>MDQITRILEKLNQQRSGETTVTLADFMPMSLAEIRSQNTGRLSREEAQLLHRAAQKEKQNNILYTARMLTRANPLLKKEMNTARYYGATPYGYDDIIPPRAEKFVAPGAVSSMFSPAGYLTELYREARGLHPKDSDRNLDKRRQDLAKLVLSQDNLDNEISALSLANEQLETALMAQTGKTDKNKYYETLATSRRSGVTPYNAPFEGIHNALAQRNFVLPDNILSNPAKFAILAAYDAGISPKLYNILTEDTESLTGSDLENSLKRNFPKVKIKDLMTLDALANYYELPADDIQALIAAEITGRLPTPDVYNDDNKLVIPAINTGGKITFSELAKTQSDEKQADYIDLIPQGGNQFLVNFSVKKTKKDATHFSIGYNKSFNNLADKNGFVPLAGEHYSIPVTLDAKILEKKTKIGITRKKPEPASDENHYTSATFTIHPNAEPGIWLLRLNKTLRLAKVSGMTPHETQHALIHVRNDSSEYELRRFTETLLYRKRYGIDTETALMLCNAGISRISYDGQLSHFDRLFNNPPLNGVTYTLGGDDILMEPDAGDPRREVLKRAFRVDNTGLWQLLVITNRENKSKTIENKTEKLRGLLFVRLLADVHNLTVAQLDALLQISPYNSMNVYALDGKTRQKMLSFLSRITQWLNTQNITVEQLMLLLDKISPAAPTKEMQVLLDLLRNGGIDKTNTKTLYTTMAPVITAAMQLDITESGEALLRWLDNNHPAGILTTSEARKLIIKKGQTAGDKEKLAAWCQALAQRVLVIRTFTLSNAELQTLSQGAPAGTITELYNISDFHNLINRCGEQAGTVLDALQSGTLTVKILAQALNLSEEVITQALTLAGQKPELTTWAQLAVLPPRLDLADTLHITPKDITTLLTVSENVRPFYTDLSALAGLLQAGLNEQQTKQLQNQSEPRRNEALSGEYRSLVMNNPVADRDDIWRNLLVDGKVSAEITTTLLADAIAGIQLYINRTIAGDEPGADSDALERQFFKDWDACNKRYSTWAGVSQLVYYPENFVDPTLRTGQTGMMNTMLEQLSQSELNKDTLENGFRQYLTAFEQVADLKVVSGYHDTVNINQGNTWFIGTSQTEPKKYYWRKADHSKCQNGRFAANAWSDWKEITCAVNPYGDMVRPVIFHSRLYLLWIEKQVQKDNTGKDTASFTLKLTHVKYDGSWASPFSYDITEKNISGWKKTGLYCAASQEDNSLLIAWYQIEKETQPNSFGLHIQPDMSCKKEPNIAGILATVTHQLDTETTVRVNTLLNRISSFEFTLEKQEGNKEIDLVISHGDYTVKTENSISALILNPTAYINITPYKLFSDIPDFYREKYITHLNSHSGTVYAPESKKMEPANNAISDKVNACAVYTYN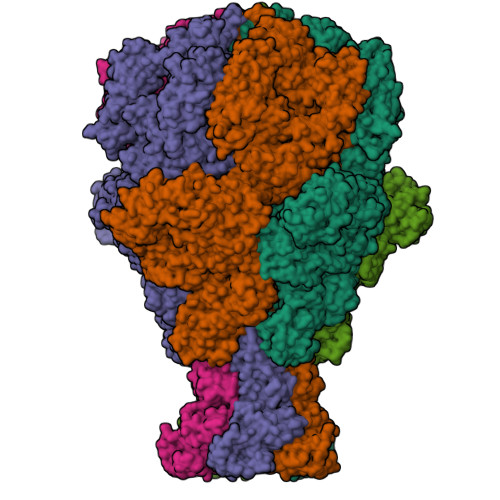NKPPKKHISLSIGKNYPLITPLELVGRKLESFFIKHKETSALYYTYGDATDDRLTLEEDKYTISTGEKKLGTLSLGKMIAQVKTISSDDISMEIELNSTKFETITGSDVGLRPPLYPTVSRETLAFPFGKLSITIPAGADINNLDCTIKVRFKNTDVLAATTTYKLVIKKTDPVQKVISLYTTPDGAQYMEWDGYRTRLNTLFTRQLIERANNGIDAILSPETQYLPEPKPGQGTYVTLILKPYDKNTHGTNRAFTIYYSNDATGSGKFPVYSGSLSVTDNTEVKLFIPLIKPGKNAVSQSAGAQQDTLYLNATYQKEATKQILLFRTDNNPEGWTLDKSVNNGTFAGLAENGVTGLLQSGEPMDFSGANALYFWELFYYTPMMVATRLLQEQNFTEANRWLSYIWQPAASGAGDWRVRPLKEDTSWNADPLDSVDPDAVAQNDPMHYKVSTLMKLLDLLIARGDKAYRMQERDTLNEAKMWYMQALGLLGDKPVSIFSNGWENPSLSNAADKTQAKQFHDEISRIRSGGLLPDVRTANTLTGLFRPQQNEKLLGYWQMLEMRLFNLRNNLSIDGQPLSLPVFAAPADPAALLSAAAAASGGSKPLPSADIPAMRFPQALDSARSLTGQLMQFGSTLLGLIERRDAEAMSELLQNQAGELMLSSLRMQEQALTELDAEKKILEQSRAGAQSRVDSYRALYDENVSAEEKRTMDLYLSSAILSTSIGVLDMAAAAADMAPNIFGVAVGGSRWGGIPKAIGAGMSLAASATKITADNISQSEAWRRRRQEWEIQKNNAESEIRQIDAQLEALAVRRTATEMQREHMEIQQAQTQAQLEFLQRKFSNKALYSWLRGRLASIYYRFYDLTAARCMMAEKAYAWQTNDTATRYIKSGAWQSNNAGLMAGESLLLNLAEMEQAWLKRDSRSLEVTRTVSLAAVYRTDNVTLAEGIADLLKGNGSGNIPASTGLSMTADNQLHAAFNLKALNIKDDYPEALGTTRRIKQISVTLPALVEPYQDMRAIFRYGGNSLPAGCKAIALSHGINDDGLFRLDFNDGRWLPFEGIPVDDDNSLTLSFPDATGEKQKPLLLSLTDIIIHIRYTIC[5x]> GMEERRQKFYPEEELVALVRSLDRPQDEGLFSMDVLVVYPHLEQEYTRVCPKRCDLATAAEKAA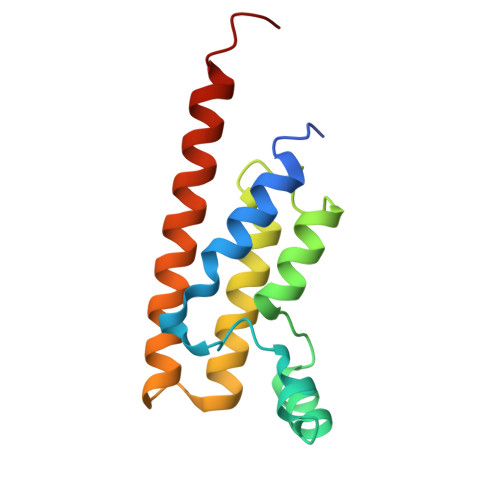NEAYSYDVNLTALREDIKLMVNNCYRFNGTKGPLANIAERFEAFAKEQIDAYVTKKAGGRRLSSLRL> GGGRPTEIENINPNVYDRIKERVLTANEEDENVPDPFDKREIFDLIRNINDPEHPLTLEELHVVQEDLIRINDSQNSVHISFTPTIPHCSMATLIGLSIRVKLLRSLPPRFKVTVEITPGTHASELAVNKQLADKERVAAALENNHLAEVIN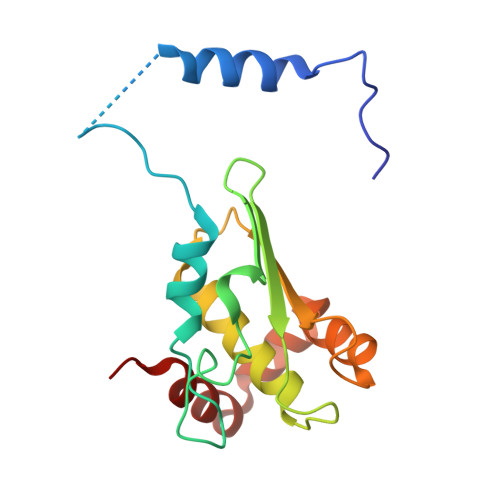QCIAAKG> GPVCAEASDVYSPCMIASTPPAPFSDVTAVTFDLINGKITPVGDDNWNTHIYNPPIMNVLRTAAWKSGTIHVQLNVRGAGVKRADWDGQVFVYLR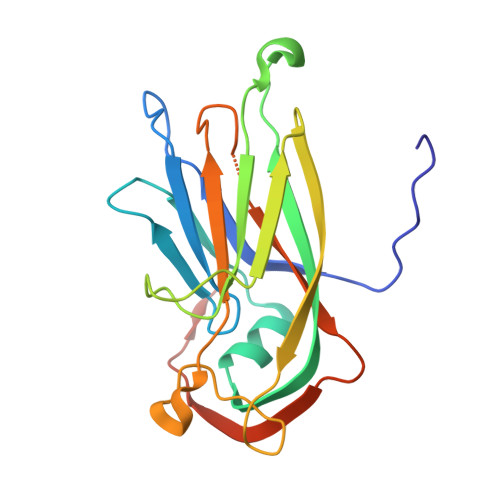QSMNPESYDARTFVISQPGSAMLNFSFDIIGPNSGFEFAESPWANQTTWYLECVATNPRQIQQFEVNMRFDPNFRVAGNILMPPFPLSTETPPL> MAFSELLDLVGGLGRFQVLQTMALMVSIMWLCTQSMLENFSAAVPSHRCWAPLLDNSTAQASILGSLSPEALLAISIPPGPNQRPHQCRRFRQPQWQLLDPNATATSWSEADTEPCVDGWVYDRSIFTSTIVAK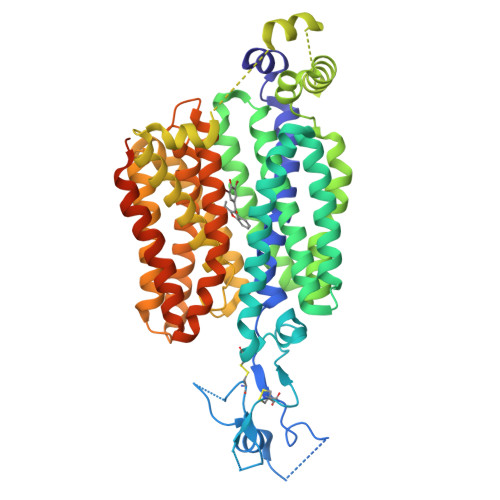WNLVCDSHALKPMAQSIYLAGILVGAAVCGPASDRFGRRLVLTWSYLQMAVSGTAAAFAPTFPVYCLFRFLLAFAVAGVMMNTGTLLMEWTSARARPLVMTLNSLGFSFGHGLTAAVAYGVRDWTLLQLAVSVPFFLCFLYSWWLAESARWLLTTGRLDRGLQELRRVAAINGKRAVQDTLTPEVLLSAMREELSVGQAPASLGTLLRTPGLRLRTCISTLCWFAFGFTFFGLALDLQALGSNIFLLQVLIGVVDIPAKMGALLLLSRLGRRPTLAASLLLAGLCILANTLVPHEMGALRSALAVLGLGGVGAAFTCITIYSSELFPTVLRMTAVGLGQMAARGGAILGPLVRLLGVHGPWLPLLVYGTVPVLSGLAALLLPETQSLPLPDTIQDVQNQAVKKATHGTLGNSVLKSTQF> QENRLLNESESSSQGLLGYYFSDLNFQAPMVVTSSTTGDLSIPSSELENIPSENQYFQSAIWSGFIKVKKSDEYTFATSADNHVTMWVDDQEVINKASNSNKIRLEKGRLYQIKIQYQRENPTEKGLDFKLYWTDSQNKKEVISSDNLQLPELKQKSSNSLEVLFQGSTSAGPTVPDRDNDGIPDSLEVEGYTVDVKNKRTFLSPWISNIHEKKGLTKYKSSPEKWSTASDPYSDFEKVTGRIDKNVSPEARHPLVAAYPIVHVDMENIILSKNEDQSTQNTDSQTRTISKNTSTSRTHTSEVHGNAEVHASFFDIGGSVSAGFSNSNSS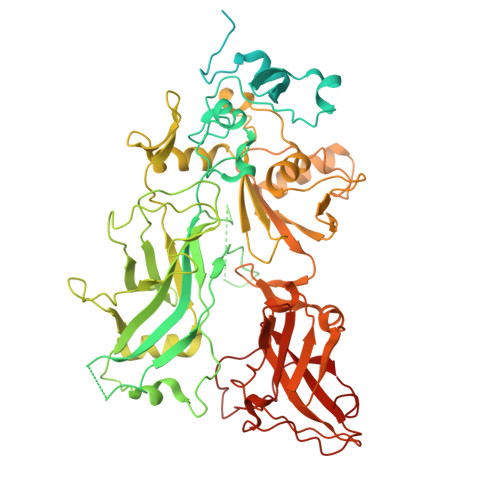TVAIDHSLSLAGERTWAETMGLNTADTARLNANIRYVNTGTAPIYNVLPTTSLVLGKNQTLATIKAKENQLSQILAPNNYYPSKNLAPIALNAQDDFSSTPITMNYNQFLELEKTKQLRLDTDQVYGNIATYNFENGRVRVDTGSNWSEVLPQIQETTARIIFNGKDLNLVERRIAAVNPSKPLETTKPDMTLKEALKIAFGFNEPNGNLQYQGKDITEFDFNFDQQTSQNIKNQLAELNATNIYTVLDKIKLNAKMNILIRDKRFHYDRNNIAVGADESVVKEAHREVINSSTEGLLLNIDKDIRKILSGYIVEIEDTEGLKEVINDRYDMLNISSLRQDGKTFIDFKKYNDKLPLYISNPNYKVNVYAVTKENTIINPSENGDTSTNGIKKILIFSKKGYEIG> ETPPRFTRTPVDQTGVSGGVASFICQATGDPRPKIVWNKKGKKVSNQRFEVIEFDDGSGSVLRIQPLRTPRDEAIYECVASNNVGEISVSTRLTVLREDQIPRGFPTIDMGPQLKVVERTRTATMLCAASGNPDPEITWFKDFLPVDTSNNNGRIKQLRSESIGALQIEQSEESDQGKYECVATNSA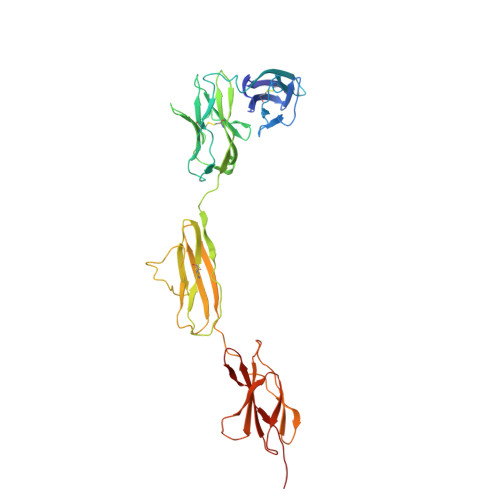GTRYSAPANLYVRVRRVPPRFSIPPTNHEIMPGGSVNITCVAVGSPMPYVKWMLGAEDLTPEDDMPIGRNVLELNDVRQSANYTCVAMSTLGVIEAIAQITVKALPKPPGTPVVTESTATSITLTWDSGNPEPVSYYIIQHKPKNSEEPYKEIDGIATTRYSVAGLSPYSDYEFRVVAVNNIGRGPASEPVLTQKHHHH> MARGLQGVMLRSFGARDHTATVIETISIAPHFVRVRMVSPTLFQDAEAEPAAWLRFWFPDPNGSNTEFQRAYTISEADPAAGRFAVDVVLHDPAGPASSWARTVKPGATIAVMSLMGSSRFDVPEEQPAGYLLIGDSASIPGMNGIIETVPNDVPIEMYLEQHDDNDTLIPLAKHPRLRVRWVMRRDEKSLAEAIENRDWSDWYAWATPEAAALKCVRVRLRDEFGFPKSEIHAQAYWNAGRAMGTHRATEPAATEPEVGAAPQPESAVPAPARGSWRAQAASRLLAPLKLPLVLSGVLAALVTLAQLAPFVLLVELSRLLVSGAGAHRLFTVGFAAVGLLGTGALLAAALTLWLHVIDARFARALRLRLLSKLSRLPLGWFTSRGSGSIKKLVTDDTLALHYLVTHAVPDAVAAVVAPVGVLVYLFVVDWRVALVLFGPVLVYLTITSSLTIQSGPRIVQAQRWAEKMNGEAGSYLEGQPVIRVFGAASSSFRRRLDEYIGFLVAWQRPLAGKKTLMDLATRPATFLWLIAATGTLLVATHRMDPVNLLPFMFLGTTFGARLLGIAYGLGGLRTGLLAARHLQVTLDETELAVREHPREPLDGEAPATVVFDHVTFGYRPGVPVIQDVSLTLRPGTVTALVGPSGSGKSTLATLLARFHDVERGAIRVGGQDIRSLAADELYTRVGFVLQEAQLVHGTAAENIALAVPDAPAEQVQVAAREAQIHDRVLRLPDGYDTVLGANSGLSGGERQRLTIARAIL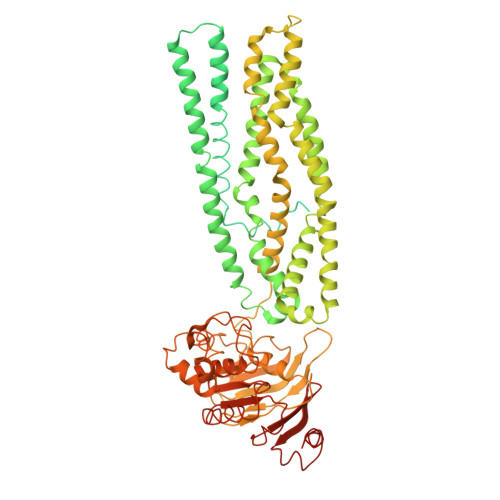GDTPVLILDQATAFADPESEYLVQQALNRLTRDRTVLVIAHRLHTITRADQIVVLDHGRIVERGTHEELLAAGGRYCRLWDTGQGSRVAVAAAQDGTR>MQSINFRTARGNLSEVLNNVEAGEEVEITRRGREPAVIVSKATFEEWHHHHHH[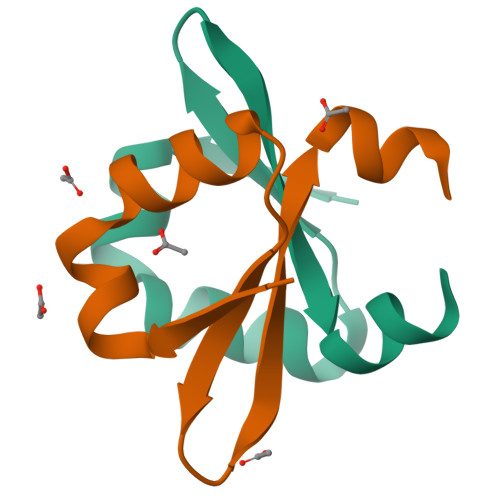2x]> XISIDEKLLQASGILEYEKVQVVNVNNGARFETYTIATQEEGVVCLNGAAARLAEVGDKVIIMSYADFNEEEAKTFKPKVVFVDENNTATKITNYEKHGA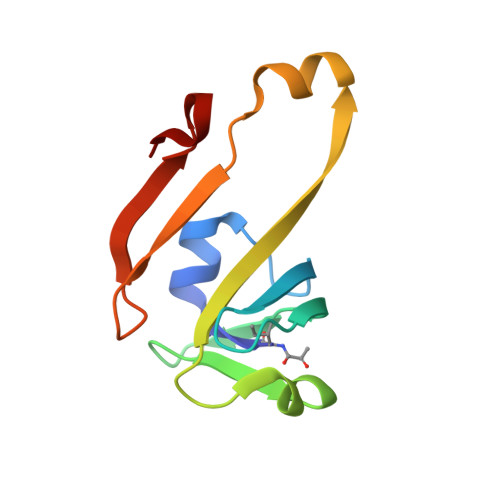IF(2R,4S)-2-[(1R)-1-{[(2,6-dimethoxyphenyl)carbonyl]amino}-2-oxoethyl]-5,5-dimethyl-1,3-thiazolidine-4-carboxylic 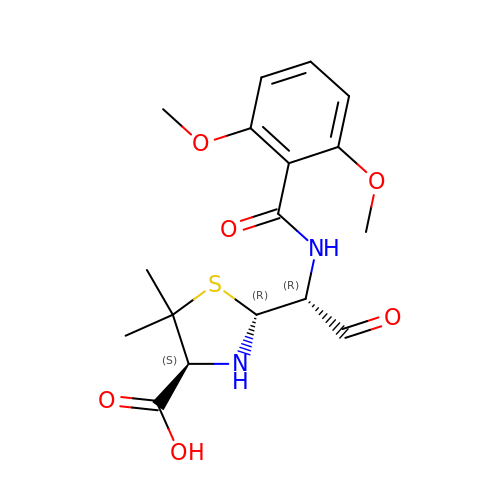acid | C17 H22 N2 O6 S | SKOKQNRJVBPEBM-ZDBHGNHJSA-N[[(2~{R},3~{S},4~{R},5~{R})-5-(6-aminopurin-9-yl)-3,4-bis(oxidanyl)oxolan-2-yl]methoxy-oxidanyl-phosphoryl] [(2~{R},3~{S},4~{S})-5-[5-[(~{E})-4-carbamimidamidobut-2-enoyl]-7,8-dimethyl-2,4-bis(oxidanylidene)-1~{H}-benzo[g]pteridin-10-yl]-2,3,4-tris(oxidanyl)pentyl] hydrogen phosphate | C32 H42 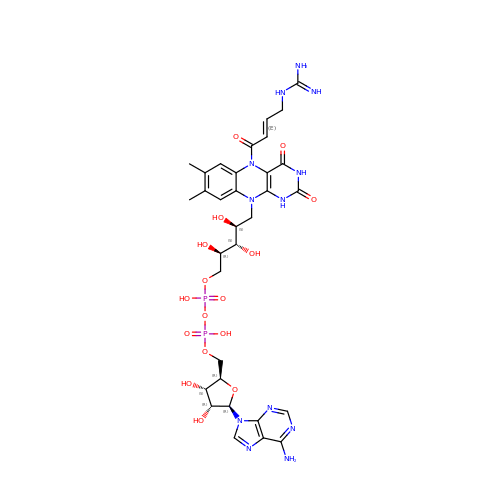N12 O16 P2 | UNPAMCKSCHHHHK-IGVXTPOKSA-N>UCAAUGGUACGGUACUUCCAUUGUCAUGUGUAUGUUGGGGAUUAAACCCUGAUUGAGUUCAGCCCACAUACUUUGUUGAUUGGUUGUCAAUCAUG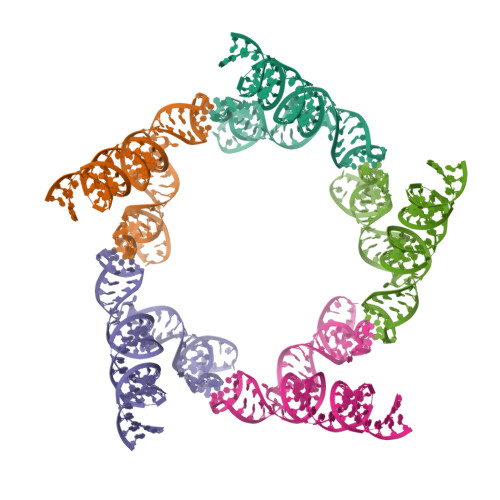GCAAAAGUGCACGCUACUUUGAUAA[5x]> MIKSALLVLEDGTQFHGRAIGATGSAVGEVVFNTSMTGYQEILTDPSYSRQIVTLTYPHIGNVGTNDADEESSQVHAQGLVIRDLPLIASNFRNTEDLSSYLKRHNIVAIADIDTRKLTRLLREKGAQNGCIIAGDNPDAALALEKARAFPGLNGMDLAKEVTTAEAYSWTQGSWTLTGGLPEAKKEDELPFHVVAYDFGAKRNILRMLVDRGCRLTIVPAQT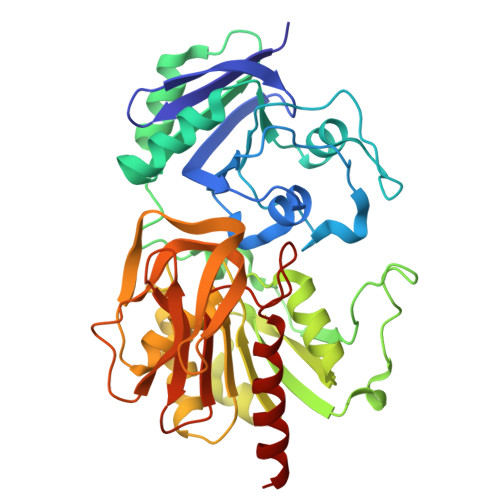SAEDVLKMNPDGIFLSNGPGDPAPCDYAITAIQKFLETDIPVFGISLGHQLLALASGAKTVKMKFGHHGGNHPVKDVEKNVVMITAQNHGFAVDEATLPANLRVTHKSLFDGTLQGIHRTDKPAFSFQGHPEASPGPHDAAPLFDHFIELIEQYRKTAK> MVAKSAALVVMGLSMASAFLAPTPNNRASAQAPMKMAKSAATKEFPFDDQPGGVKWFPSSAPYWDPLGFTNEKTEDEYWRIAHGEIKNGRLAMLAVTHYFVVGSGLRFPFKFGSVSTADVPLGLGAIKALPWAVWLQIAAFCLVLEVLTENPG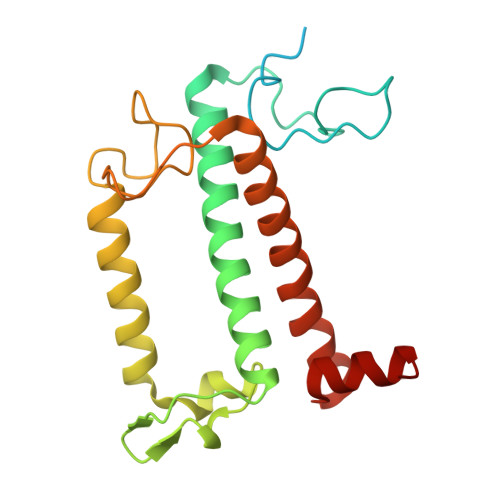FGERVPGRVPGNLQPDTPSFNAPGDLEIRTKELNNARLAMISIWGLWVGEIASGGVDPFTSFANWLKL>DALKVNRAPVGVEPQEVHKWLQSFNWDFKENRTKYPTKYHMANETKEQFKVIAKEYARMEAAKDERQFGTLLDGLTRLGAGNKVHPRWGETMKVISNFLEVGEYNAIAASAMLWDSATAAEQKNGYLAQVLDEIRHTHQCAFINHYYSKHYHDPAGHNDARRTRAIGPLWKGMKRVFADGFISGDAVECSVNLQLVGEACFTNPLIVAVTEWASANGDEITPTVFLSVETDELRHMANGYQTVVSIANDPASAKFLNTDLNNAFWTQQKYFTPVLGYLFEYGSKFKVEPWVKTWNRWVYEDWGGIWIGRLGKYGVESPASLRDAKRDAYWAHHDLALAAYAMWPLGFARLALPDEEDQAWFEANYPGWADHYGKIFNEWKKLGYEDPKSGFIPYQWLLANGHDVYIDRVSQVPFIPSLAKGTGSLRVHEFNGKKHSLTDDWGERQWLIEPERYECHNVFEQYEGRELSEVIAEGHGVRSDGKTLIAQPHTRGDNLWTLEDIKRAGCVFPDPLAKF[2x];>PQSSQVTKRGLTDPERAAIIAAAVPDHALDTQRKYHYFIQPRWKRLSEYEQLSCYAQPNPDWIAGGLDWGDWTQKFHGGRPSWGNESTELRTTDWYRHRDPARRWHHPYVKDKSEEARYTQRFLAAYSSEGSIRTIDPYWRDEILNKYFGALLYSEYGLFNAHSSVGRDCLSDTIRQTAVFAALDKVDNAQMIQMERLFIAKLVPGFDASTDVPKKIWTTDPIYSGARATVQEIWQGVQDWNEILWAGHAVYDATFGQF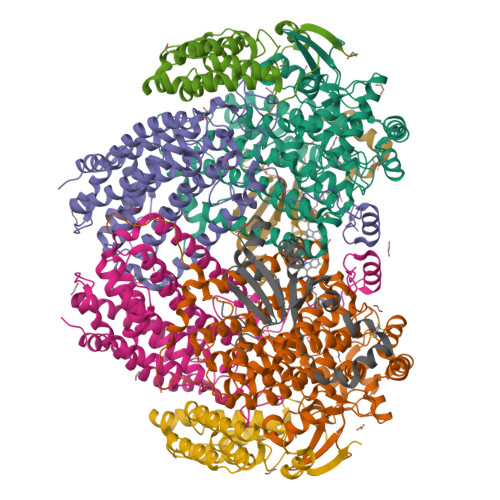ARREFFQRLATVYGDTLTPFFTAQSQTYFQTTRGAIDDLFVYCLANDSEFGAHNRTFLNAWTEHYLASSVAALKDFVGLYAKVEKVAGATDRAGVSEALQRVFGDWKIDYADKIGFRVDVDQKVDAVLAGYKN[2x];>[2x]AKREPIHDNSIRTEWEAKIAKLTSVDQATKFIQDFRLAYTSPFRKSYDIDVDYQYIERKIEEKLSVLKTEKLPVADLITKATTGEDAAAVEATWIAKIKAAKSKYEAERIHIEFRQLYKPPVLPVNVFLRTDAALGTVLMEIRNTDYYGTPLEGLRKERGVKVLHLQA;>SAHNAYNAGIMQCTGKAFADEFFAEENQVVHESNAVVLVLMKSDEIDAIIEDIVLKGGKAKNPSIVVEDKAGFWWIKADGAIEIDAAEAGELLGKPFSVYDLLINVSSTVGRAYTLGTKFTITSELMGLDRALTDI[2x]>[2x]SNAETIEIIKDLFEHLCGVRVHRTYEDDTGLWFDTSQGSKNGIMDYKLGFVKSQAENTTEVDTEVIYVPLLKQRTAEELQELQKKLPDYLFETLSFPLRSLNQFYIKMSKSLNKKV;> GDKDNGLHAGETDGDDEGFEFRRHSNLGVPTLGERLDSLHEIKSARRMDHFNSSRNSLR

In S. cerevisiae meiosis I, sister kinetochores are fused through the action of the kinetochore-binding monopolin complex, and together bind a single microtubule. The conserved core of the monopolin complex comprises two nucleolar proteins, Csm1 and Lrs4. These proteins form a distinctive V-shaped complex, with two Csm1 homodimers bridged at their coiled-coil N-termini by a pair of Lrs4 subunits, thereby positioning two pairs of Csm1 globular-domain “heads” ~ 10 nm apart at the apices of the V. Each Csm1 globular domain has a conserved hydrophobic cavity implicated in binding the kinetochore protein Dsn1, leading to the proposal that monopolin could bridge Dsn1 molecules from sister kinetochores to physically fuse the kinetochores. A ~ 40-residue region within the disordered N-terminus of the core kinetochore protein, Dsn1, has been identified as the kinetochore receptor for the monopolin subunit Csm1.

We therefore screened paralogs from several related budding yeast, and successfully purified a complex between the Candida glabrata (Cg) Csm1 globular domain (residues 69–181) and the Dsn1 Box 1-2-3 region (residues 14–72). We identified crystallisation conditions for this complex and determined the structure to 2.3 Å resolution. Our structures of the Cg Csm169–181:Dsn114–72 and Cg Csm169–181:Sc Dsn171–110 complexes reveal a consistent interface between Dsn1 Box 2-3 and Csm1, while the Cg Csm169–181:Dsn114–72 structure reveals a second interface between Csm1 and Dsn1 Box 1. In the crystal structures of both Cg Csm169–181:Dsn114–72 and the chimeric Cg Csm169–181:Sc Dsn171–110 complex, the Dsn1 Box 2–3 region wraps around the Csm1 globular domain, with Box 2 forming an α-helix that packs against the “side” of the Csm1 dimer, and Box 3 binding the Csm1 hydrophobic cavity. While Dsn1 Box 2 forms an α-helix and associates with the “side” of the Csm1 dimer, Box 3 forms an extended conformation that packs tightly against the Csm1 conserved hydrophobic cavity. Our structure of the Cg Csm169–181:Cg Dsn114–72 complex shows how Dsn1 Box 2-3 binds Csm1, but also reveals a plausible Csm1 binding mode for Box 1. In the structure, Dsn1 Box 1 extends outward from the Csm1-Dsn1 Box 2-3 complex described above, and interacts with a crystallographic symmetry-related Csm1 monomer. Interestingly, Box 1 is oriented in the opposite direction across the Csm1 hydrophobic cavity than Box 3, with positively charged residues (Cg Dsn1 R35 and R36, equivalent to Sc Dsn1 K75 and R76) C-terminal to the hydrophobic residues, and negatively charged residues (Cg Dsn1 D29 and E30, equivalent to Sc Dsn1 S29 and P30) N-terminal. Thus, both Dsn1 Box 1 and Box 3 bind the same surface of Csm1, through similar but distinct interaction modes.>[3x]ADAAAGAQVFAANCAACHAG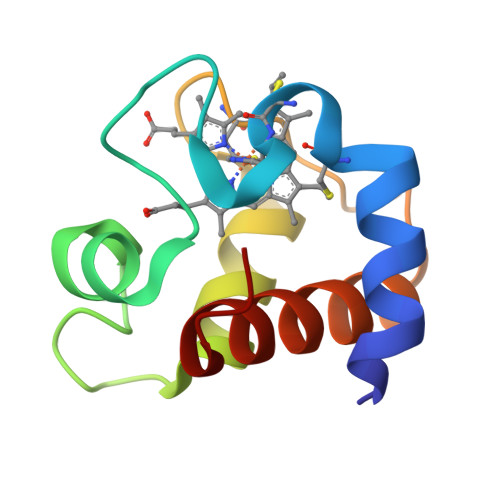GNNAVMPTKTLKADALKTYLAGYKDGSKSLEEAVAYQVTNGQGAMPAFGGRLSDADIANVAAYIADQAENNKW PHOSPHOMETHYLPHOSPHONIC ACID ADENOSYL ESTER | C11 H17 N5 O9 P2 | 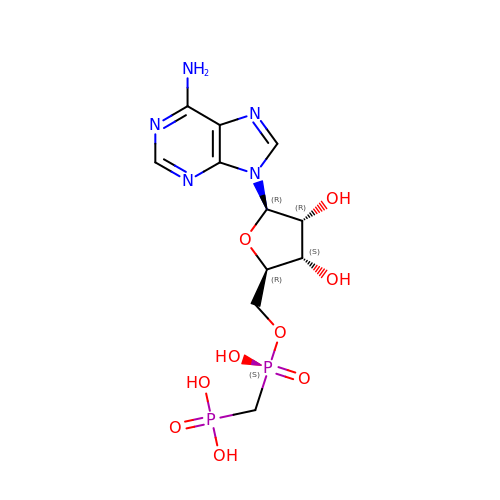OLCWZBFDIYXLAA-IOSLPCCCSA-N> SWDLVTCFCMKPFAGRPMIECNECHTWIHLSCA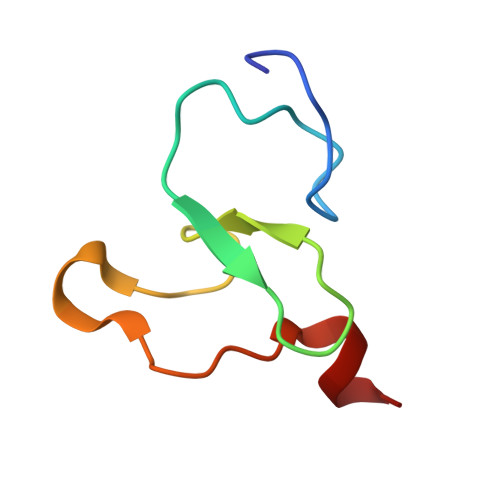KIRKSNVPEVFVCQKCRDS> FSIVGSLPR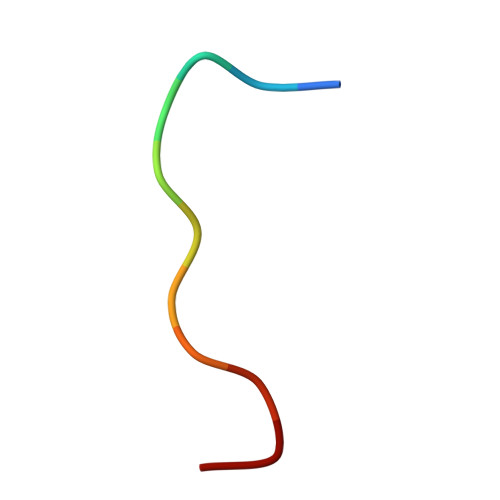DC> GSQEDFELIQRIGSGTYGDVYKARNVNTGELAAIKVIKLEPGEDFAVVQQEIIMMKDCKHPNIVAYFGSYLRRDKLWICMEFCGGGSLQDIYHVTGPLSELQIAYVSRETLQGLYYLHSKGKMHRDIKGA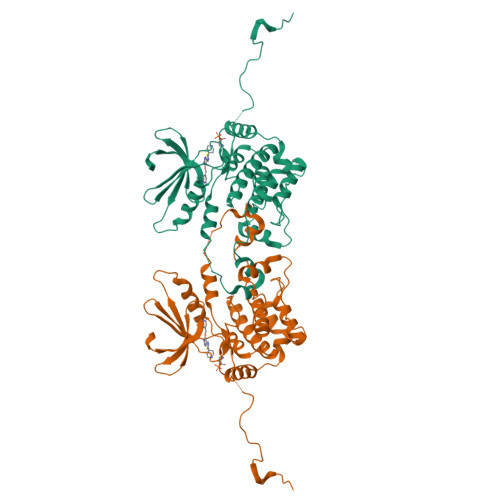NILLTDNGHVKLADFGVSAQITATIAKRKAFIGTPYWMAPEVAAVERKGGYNQLCDLWAVGITAIELAELQPPMFDLHPMRALFLMTKSNFQPPKLKDKMKWSNSFHHFVKMALTKNPKKRPTAEKLLQHPFVTQHLTRSLAIELLDKVNNPDHSTYHDFDDDDPEPLVAVPHRIHSTSRNVREEKTRSEITFGQVKFDPPLRKETEPHHELPDSDGFLDSSEEIYYTARSNLDLQLEYG5-(1~{H}-1,2,3,4-tetrazol-5-yl)quinolin-8-ol | C10 H7 N5 O | 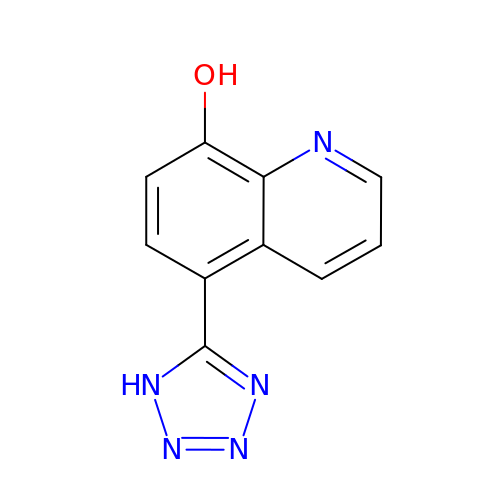COSOIVLLWHGBPW-UHFFFAOYSA-N> MYDPNTSQTEKQKQEEFLKLKIQEAFNLFVKDKKGIVDKREIPYIMRYLGQFPSEAQVRDAILPEIEEDEPSEFIKYSKFEPYMLKVLKEREYEPDDPEALLA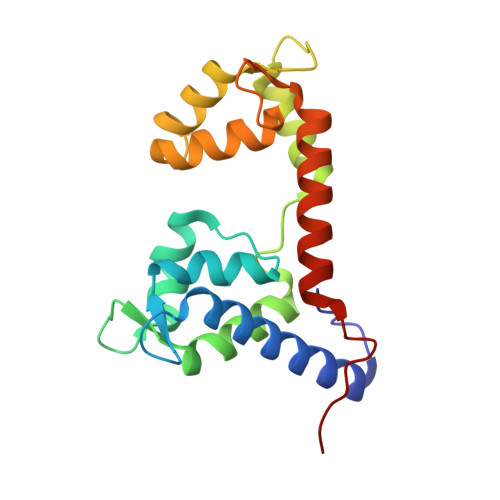AFKLLDQEGKGYIEIDMMKTFLEKQGIEFREQETKSFIEFATNKDPNATVIYYEDYISRLQAFTDKHIESVMKGYNNFQVKK α-1,3-Glucanase (E.C.3.2.1.59) hydrolyses the α-1,3-glucoside linkages in α-1,3-glucan, which is found in fungal cell walls and extracellular polysaccharides produced by oral Streptococci1,2. α-1,3-Glucanases are classified into family 71 and 87 of glycoside hydrolases (GHs) based on their amino acid sequences. GH 87-type α-1,3-glucanase was isolated from the culture filtrate of Bacillus circulans KA-304 and termed Agl-KA. Agl-KA hydrolyses the α-1,3-glucan of oral Streptococci as well as of fungi. Agl-KA is also multimodular, comprising an N-terminal discoidin domain (DS1), followed by a carbohydrate-binding module 6 (CB6), threonine and proline repeats (TP), a second discoidin domain (DS2), an uncharacterised conserved domain (UCD) and a C-terminal catalytic unit (AglΔDCD-UCD).

In this study, we successfully determined the x-ray crystal structure of AglΔDCD-UCD using the Se-MAD method. The crystal structure of AglΔDCD-UCD was determined at a resolution limit of 1.83 Å. Two molecules (molecules A and B) were positioned in the asymmetric unit and were essentially identical (root mean square deviation, 0.14 Å); hereafter, molecule A is used for discussion. Five Ca+ ions, two Zn2+ ions, two SO42− molecules and one polyethylene glycol chain were observed within one protein molecule. The positions of three Ca+ ions (out of five) were relatively buried in the protein structure, indicating these may contribute to protein stability. The overall structure of AglΔDCD-UCD comprised an N-terminal galactose-binding-like domain (~180 residues), followed by a right-handed β-helix (~400 residues), as determined based on the CATH domain classification. The striking difference between AglΔDCD-UCD and other β-helix folds of CASH is the presence of the galactose-binding-like domain, which forms a complex with the β-helix domain. The interface area between the galactose-binding-like domain and the β-helix domain was 1743 Å2, indicating that a large surface area was buried upon complex formation and the complex was stabilised. Interestingly, a Ca2+ ion is coordinated to the carboxy group of D1067, D1090 and water molecules, with pentagonal–bipyramidal coordination. The β-helix fold creates a concave surface along with the β-helix direction, resulting in a consecutive groove of the putative substrate recognition cleft.

>[2x]MSHMNLVVYAQRGASMPYTRYDTDDAARGGGATLQSAPNFDQALTASEASGQRYIALPSNGSYAQWTIRPGEGGDGVTMRFTMPDSANGMGLNGSLDVYVNGVKAKTVPLTSYYSWQYFSSDHPADTPAGGRPLFRFDEVHWKMDTPLQPGDTIRIQKSGADSLEYGVDFLEIEAVPAAIARPANSVSVTDFGAVANDGQDDLAAFEAAVNAAVTSGKILYIPAGTFHLGNMWKIGSVANKINNITIMGAGIWHTNIQFTNPNQASGGISFRVTGQLDFSHIYMNSNLRSRYGEQAVYKGFMDNFGTNSKVHNVWVEHFECGFWVGDYAHTPAIIANGLVIENSRIRNNLADGVNFAQGTSNSTVRNSSIRNNGDDGLAVWTSNVNGAPAGVNNTFSYNTIENNWRAAGIAFFGGSGHKATHNLIVDTVGGSAIRMNTVFPGYHFQNNTGIVFSDTTIINSGTSRDLYNGERGAIDLEASNDPIKNVTFTNIDIINTQRSAIQFGYGGGFENIVFNNININGAGKDGVLTSRFSSPHPGAAIYTYTGNGSATFNNLTTNDIAHPNLYFIQNGFNLTIQ~{N}-[(1~{R})-2-[4-(azetidin-1-ylcarbonyl)phenyl]-1-cyano-ethyl]-3-(3,4-dimethoxyphenyl)-1,2,4-oxadiazole-5-carboxamide 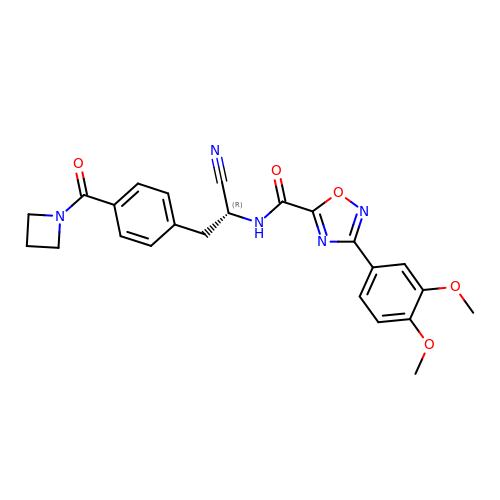| C24 H23 N5 O5 | SMNJIXFCHIEXRX-GOSISDBHSA-N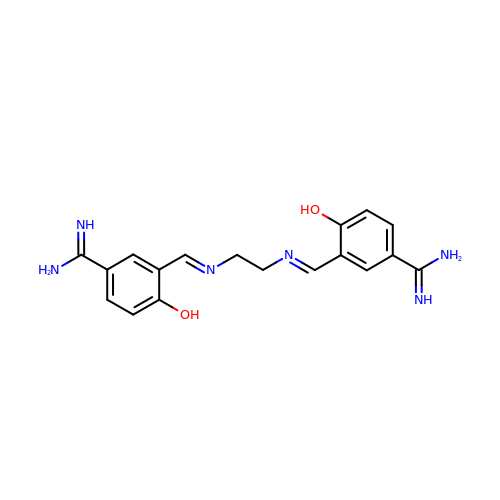3,3'-[ethane-1,2-diylbis(nitrilomethylylidene)]bis(4-hydroxybenzenecarboximidamide) | C18 H20 N6 O2 | YUJGWDWOHQDFJV-UHFFFAOYSA-N>SVKLTMWIMPNSDTPDQD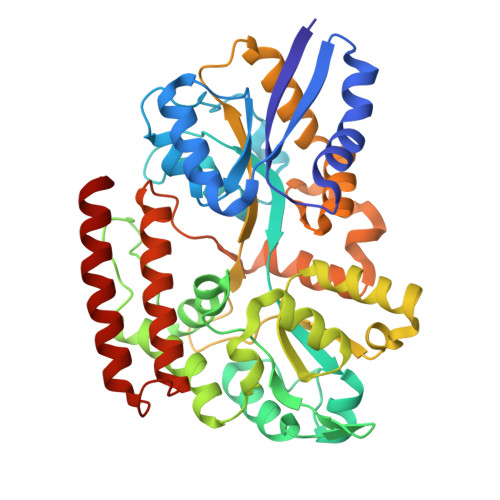LLKVVKPFTDANPHITVEPTVVDWSAALTKITAAATSGEAPDITQVGSTWTAAIGAMEGALVELTGKIDTSAFVESTLQSAYIKGTDKMFGMPWFTETRALFYRKDACEKAGVNPETDFATWDKFKDALKKLNGIEVDGKKLAALGMPGKNDWNVVHNFSWWIYGAGGDFVNEEGTQATFSSENALKGIKFYSELAVEGLMDEPSLEKNTSDIESAFGDGAYATAFMGPWVISSYTKNKEENGNDLIDKIGVTMVPEGPAGRYAFMGGSNLVIFNSSKNKDEALELLKFFASKEAQVEYSKVSKMLPVVKAAYEDPYFEDSLMKVFKEQVDKYGKHYASVPGWASAEVIFSEGLSKIWDNVMEVDGAYSYDKTVQIVKDVESQINQILQETSK[2x]> GPEFSMEDLIPLVNRLQDAFSAIGQNADLDLPQIAVVGGQSAGKSSVLENFVGRD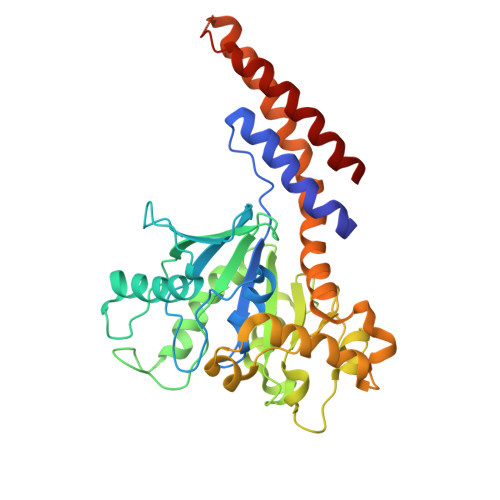FLPRGSGIVTRRPLVLQLVNATTEYAEFLHCKGKKFTDFEEVRLEIEAETDRVTGTNKGISPVPINLRVYSPHVLNLTLVDLPGMTKVPVGDQPPDIEFQIRDMLMQFVTKENCLILAVSPANSDLANSDALKVAKEVDPQGQRTIGVITKLDLMDEGTDARDVLENKLLPLRRGYIGVVNRSQKDIDGKKDITAALAAERKFFLSHPSYRHLADRMGTPYLQKVLNQQLTNHIRDTLPGLRNKLQSQLLSIEKEVEEYKNFRPDKHGTDSRVDEMLRMYHALKEALSIIGNINTTTV> MRGCGVLCAGHKRAAVIATTTCSLGPPTLSPSLTLRPVACAATPVTIPIFPPPMRGSFIDRNPVWASFNEKHTAKSFRHRIVSSADVSLRPPQFYLSNEKVSAGEAAVVQKRAEATDSYGEQLDEIS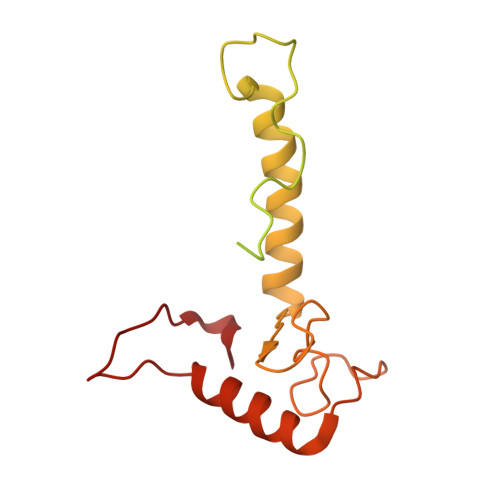ARWAAKFYGRVTFGPRNYPYPSSRWLARRFKMKKHRIIKRFRFRRYKLAAVANLPFAKMIRVGLLPELKSSKTKKGDDVEADLSGRLVSAVRSSGGKKKGNRGRPKSKYQI>MKGFIDDANYSVGLLDEGTNLGNVIDNYVYEHTLTGKNAFFVGDLGKIVKKHSQWQTVVAQIKPFYTVKCNSTPAVLEILAALGTGFACSSKNEMALVQELGVSPEN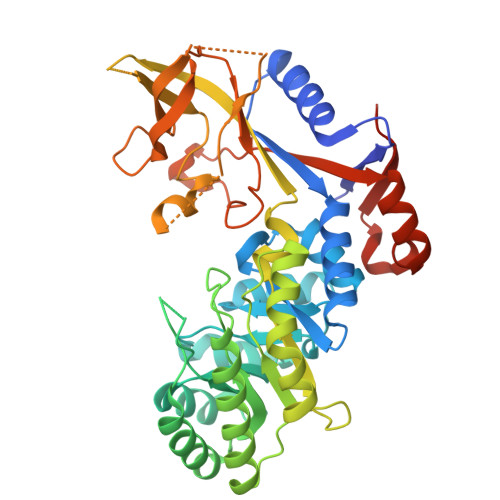IIFTSPCKQVSQIKYAAKVGVNIMTCDNEIELKKIARNHPNAKVLLHIATEDNIGGEDGNMKFGTTLKNCRHLLECAKELDVQIIGVKFHVSSACKEYQVYVHALSDARCVFDMAGEFGFTMNMLDIGGGFTGTEIQLEEVNHVISPLLDIYFPEGSGIQIISEPGSYYVSSAFTLAVNIIAKKVVENDKFSSGVEKNGSDEPAFVYYMNDGVYGSFASKLSEDLNTIPEVHKKYKEDEPLFTSSLWGPSCDELDQIVESCLLPELNVGDWLIFDNMGADSFHEPSAFNDFQRPAIYFMMSFSDWYEMQDAGITSDAMMKNFFFAPSCIQLSQEDSFSTEA[2x]> GDRVKKLINSQISLLIGKGLHEFDSLRDPEVNDFRTKMRQFCEEAAAHRQQLGWVEWLQYSFPLQLEPSARGWRAGLLRVSNRALLVNVKFEGSEESFTFQVSTKDMPLALMACALRKKATVFRQPLVEQPEEYALQVNGRHEYLYGNYPLCHFQYICSCLHSGLTPHLTMVHSSSILAMRDEQSNPAPQVQKPRAKPPPIPAKKPSSVSLWSLEQPFSIELIEGRKVNADERMKLVVQAGLFHGNEMLCKTVSSSEVNVCSEPVWKQRLEFDISVCDLPRMARLCFALYAVVEKAKKARSTKKKSKKADCPIAWANLMLFDYKDQLKTGERCLYMWPSVPDEKGELLNPAGTVRGNPNTESAAALVIYLPEVAPHPVYFPALEKILELGRHGERGRITEEEQLQLREILERRGSGELYEHEKDLVWKMRHEVQEHFPEALARLLLVTKWNKHEDVAQMLYLLCSWPELPVLSALELLDFSFPDCYVGSFAIKSLRKLTDDELFQYLLQLVQVLKYESYL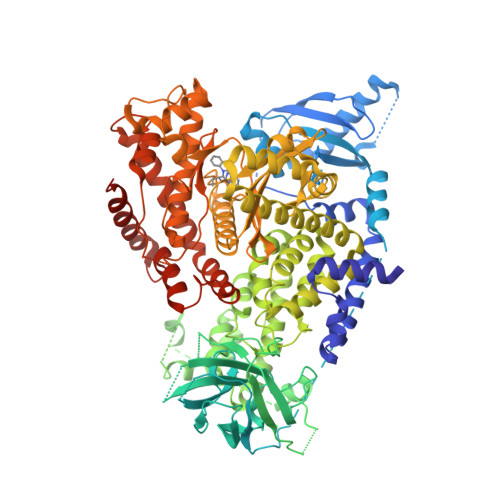DCELTKFLLGRALANRKIGHFLFWHLRSEMHVPSVALRFGLIMEAYCRGSTHHMKVLMKQGEALSKLKALNDFVKVSSQKTTKPQTKEMMHMCMRQETYMEALSHLQSPLDPSTLLEEVCVEQCTFMDSKMKPLWIMYSSEEAGSAGNVGIIFKNGDDLRQDMLTLQMIQLMDVLWKQEGLDLRMTPYGCLPTGDRTGLIEVVLHSDTIANIQLNKSNMAATAAFNKDALLNWLKSKNPGEALDRAIEEFTLSCAGYCVATYVLGIGDRHSDNIMIRESGQLFHIDFGHFLGNFKTKFGINRERVPFILTYDFVHVIQQGKTNNSEKFERFRGYCERAYTILRRHGLLFLHLFALMRAAGLPELSCSKDIQYLKDSLALGKTEEEALKHFRVKFNEALRESWKTKVNWLAHNVSKDNRQ>MRGSHHHHHHGSVIFDKRIKDEEDVEKELGLPVLGSIQKFNMTNTRRSTSSLIVHEQPKSPISEKFRGIRSNIMFANPDSAVQSIVITSEAPGAGKSTIAANLAVAYAQAGYKTLIVDGDMRKPTQHYIFNLPNNEGLSSLLLNWSTYQDSIISTEIEDLDVLTSGPIPPNPSELITSRAFANLYDTLLMNYNFVIIDTPPVNTVTDAQLFSKFTGNVVYVVNSENNNKDEVKKGKELIEATGAKLLGVVLNRMPKDKSASYYAYYGT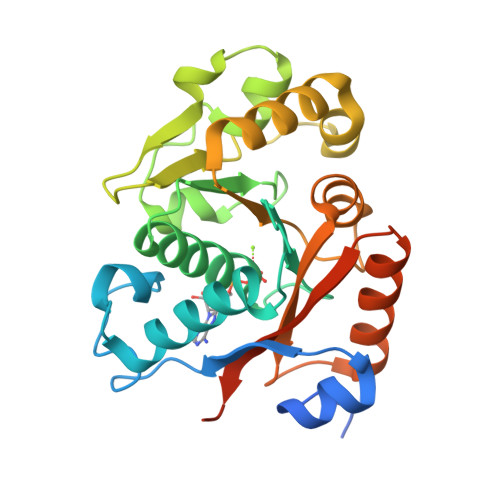DES[2x]> MPASLLRFLALAGTAVGLTTNHNHSPSCRVLPGDAAWPSSRDWAKLNKTLNGHLIATVPQASVCHKSPFGQYDAQACEELKSSWDISTITHVNAPGDVLSQNFQNYSCVPFTDPSQPCQLGNYPSYVVNVTGAADVQAALKFAQKHNVRIVIKNTGHDYLGKSTGKGALSLWMHNLKSTKFIKNYKAPYYKGPAAKLGAGVEGFEAYAMANSTGHRIVGGTCPTVGIVGGYTQGGGHSILSSSYGVAADNVLEWEVVTADGRHLVATPTRNSDLYWALSGGGGG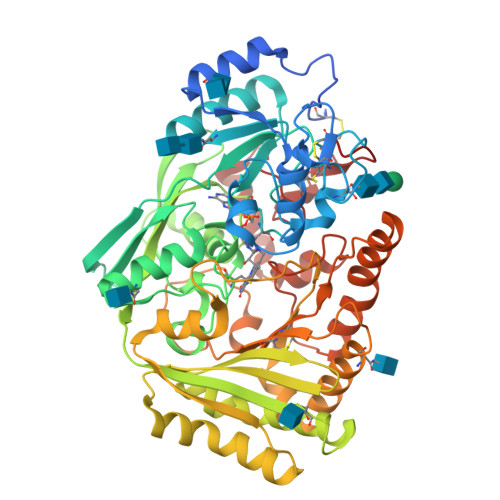TFAVVLSMTARLHRDGIVGGTLLGFNDSAVGNEVYWEAVAAFHALLPDFLDGGNSFTYSVGNNSLTAYGTMPGADRDAVDRLLRPFLDDLASRGITPVVQPRVSTNYYDHFFTYLGPAPYGNAAYFPFTNSRIIPRSLVTDPKSNAVVTDLFRNISQVPAFSPFYCDSFSVADKPHPANSLHPAWRTGMLLCAPAGSWDWDASPEEMAARDRYAAETLQPMMDAATPGGSVYLNEANHLYANWKESFYGDNYARLLRVKKKYDPDSVFYVKTGVGSEVWDVDATGRLCRA>[2x]MSQLEHNIGLSIFEPVAKHRANRIVCTIGPSTQSVEALKNLMKSGMSVARMNFSHGSHEYHQTTINNVRAAAAELGLHIGIALDTKGPEIRTGLFKDGEVSFAPGDIVCVTTDPAYEKVGTKEKFYIDYPQLTNAVRPGGSIYVDDGVMTLRVVSKEDDRTLKCHVNNHHRLTDRRGINLPGCEV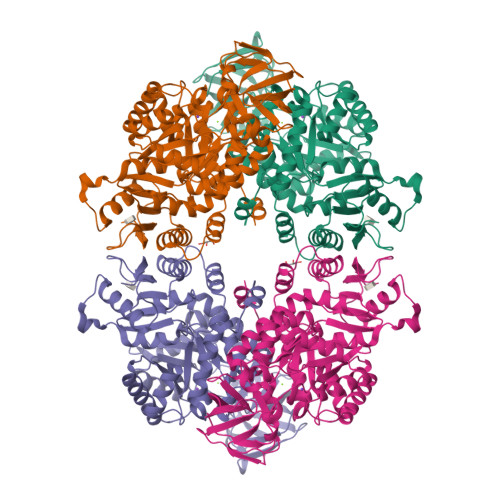DLPAVSEKDRKDLEFGVAQGVDMIFASFIRTAEQVREVRAALGEKGKDILIISKIENHQGVQNIDSIIEASNGIMVARGDLGVEIPAEKVCVAQMCIISKCNVVGKPVICATQMLESMTSNPRPTRAEVSDVANAVLNGADCVMLSGETAKGKYPNEVVQYMARICVEAQSATHDTVMFNSIKNLQKIPMCPEEAVCSSAVASAFEVQAKAMLVLSNTGRSARLISKYRPNCPIICVTTRLQTCRQLNVTRSVVSVFYDAAKSGEDKDKEKRVKLGLDFAKKEKYASTGDVVVVVHADHSVKGYPNQTRLIYLP>[6x]GMKPLKEVVGAYLALSDAQRQLVAGEYDEAAANCRRAMEISHTMPPEEAFDHAGFDAFCHAGLAEALAGLRSFDEALHSADKALHYFNRRGELNQDEGKLWI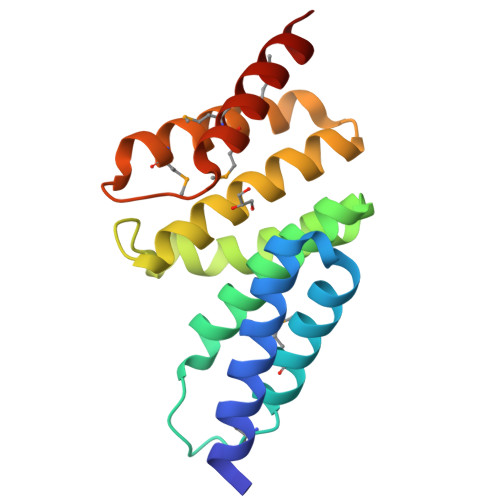SAVYSRALALDGLGRGAEAMPEFKKVVEMIEERKGETPGKERMMEVAIDRIAQLGAS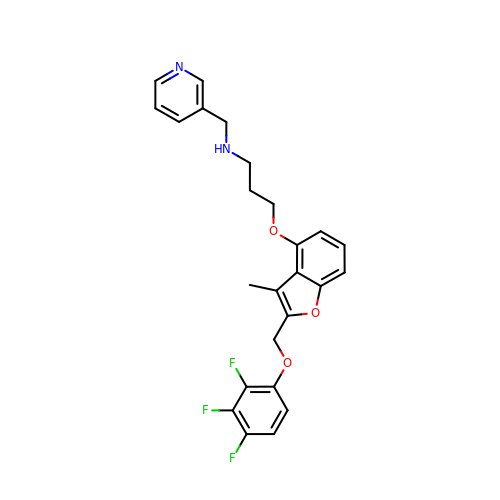3-[[3-methyl-2-[[2,3,4-tris(fluoranyl)phenoxy]methyl]-1-benzofuran-4-yl]oxy]-N-(pyridin-3-ylmethyl)propan-1-amine | C25 H23 F3 N2 O3 | FKIAZUIISXQFHC-UHFFFAOYSA-N>[2x]GS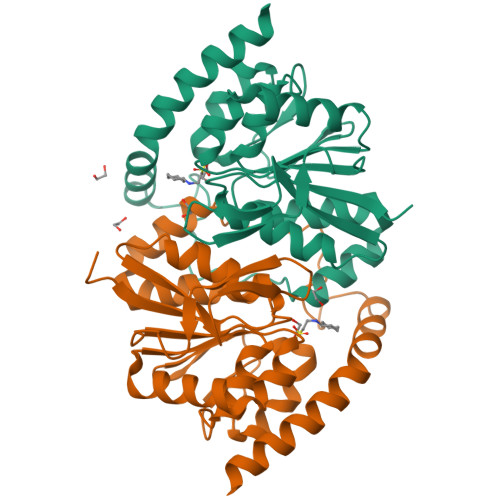HMAVQIGFLLFPEVQQLDLTGPHDVLASLPDVQVHLIWKEPGPVVASSGLVLQATTSFADCPPLDVICIPGGTGVGALMEDPQALAFIRQQAARARYVTSVSTGSLVLGAAGLLQGKRATTHWAYHELLAPLGAIPVHERVVRDGNLLTGGGITAGIDFALTLAAELFDAATAQRVQLQLEYAPAPPFNAGSPDTAPASVVQQARQRAADSLHKRREITLRAAARLAAG During infection of mammalian hosts, African trypanosomes thwart immunity using antigenic variation of the dense Variant Surface Glycoprotein (VSG) coat, accessing a large repertoire of several thousand genes and pseudogenes, and switching to antigenically distinct copies. In the salivary glands of the fly, the pathogen adopts the metacyclic form and expresses a limited repertoire of VSG genes specific to that developmental stage. We present here three novel metacyclic form VSG N-terminal domain crystal structures (mVSG397, mVSG531, and mVSG1954) and show that they mirror closely in architecture, oligomerization, and surface diversity the known classes of bloodstream form VSGs. The VSG protein can be roughly divided into three functional units: the signal peptide for delivery to the cell surface (and which is cleaved during translocation), a large N-terminal domain (NTD) that forms the bulk of the molecule, and the smaller C-terminal domain (CTD) that is tethered to the NTD by a flexible linker that can often be removed by endogenous and exogenous proteases.

We also crystallized mVSG531, predicted to be of the Class A2 group, determining its structure to 1.95Å resolution. Consistent with bioinformatic analyses, mVSG531 is very similar to the structures of other Class A2 members solved from BSF VSGs, particularly VSG1 and VSG2, aligning to each with a RMSD of 2.1Å over 354 residues and 2.4Å over 347 residues, respectively. In fact, with 35% sequence identity, the structure of VSG1 is similar enough to mVSG531 that we were able to use it to phase the diffraction data through molecular replacement. Most of the divergence between VSG531 and VSG1/VSG2 occurs in the top lobes, with the bottom lobe showing higher conservation, and the three-helix bundle the most conserved region of the molecule (RMSD close to 1Å). The positions of the two cysteine disulfides bonds in the top lobe of the N-terminal domain closely overlap with several of those in structures of bloodstream Class A2 members, although this does not hold for all Class A members, such as A3 member VSG13 and Class A1 mVSG397 and VSGsur. The N-linked sugars of VSG1, VSG2, and mVSG531 are located in very similar positions in the lower lobe as well. (A) Eight molecules of mVSG531 was found in the crystal asymmetric unit. (B) N-linked glycan is attached at Asn295 at the dimer’s bottom lobe (salmon pink spheres). Two disulfide bonds are observed at the top lobe of each molecule (green spheres).

>[2x]VNGAGLLQTVWGPVCELTSELDGQAGAALKKEQEMLAKINDMQMAQLRAAIYLAKNPSTPHQNALAVLTAYYAERAGSGKAYFLHALPKAVDSIRRAAYLKGHLDEYLNLLEKSSGGNNKCLVTTDDATVATRGGDQKLAGKNCKLSLSPLKPVDAALTYITKAGVGKLRYDDGGAGGNAVTPSKSGVHACKLLIAHNTAGYGDGGGVTADIDVFAGYMKVKATDAEPKLAAKSDLEEGGGGGAEAWKALHTAIKQEADAEAAELTNETGKLGERRHFLAAATNVLGTGAAGTGNAGRAAVEAAFGSDSEGGDRKIIELIEKELIVKGTANRDADESLGNIKTLKELGELLSYFQLKNSNTINELRNKLKA;>[3x]VNGAGLLQTVWGPVCELTSELDGQAGAALKKEQEMLAKINDMQMAQLRAAIYLAKNPSTPHQNALAVLTAYYAERAGSGKAYFLHALPKAVDSIRRAAYLKGHLDEYLNLLEKSSGGNNKCLVTTDDATVATRGGDQKLAGKNCKLSLSPLKPVDAALTYITKAGVGKLRYDDGGAGGNAVTPSKSGVHACKLLIAHNTAGYGDGGGVTADIDVFAGYMKVKATDAEPKLAAKSDLEEGGGGGAEAWKALHTAIKQEADAEAAELTNETGKLGERRHFLAAATNVLGTGAAGTGNAGRAAVEAAFGSDSEGGDRKIIELIEKELIVKGTANRDADESLGNIKTLKELGELLSYFQLKNSNTINELRNKLK;>[3x]VNGAGLLQTVWGPVCELTSELDGQAGAALKKEQEMLAKINDMQMAQLRAAIYLAKNPSTPHQNALAVLTAYYAERAGSGKAYFLHALPKAVDSIRRAAYLKGHLDEYLNLLEKSSGGNNKCLVTTDDATVATRGGDQKLAGKNCKLSLSPLKPVDAALTYITKAGVGKLRYDDGGAGGNAVTPSKSGVHACKLLIAHNTAGYGDGGGVTADIDVFAGYMKVKATDAEPKLAAKSDLEEGGGGGAEAWKALHTAIKQEADAEAAELTNETGKLGERRHFLAAATNVLGTGAAGTGNAGRAAVEAAFGSDSEGGDRKIIELIEKELIVKGTANRDADESLGNIKTLKELGELLSYFQLKNSNTINELRNKLKAV> SPVAGQKYDYILVGGGTAACVLANRLSADGSKRVLVLEAGPDNTSRDVKIPAAITRLFRSPLDWNLFSELQEQLAERQIYMARGRLLGGSSATNATLYHRGAAGDYDAWGVEGWSSEDVLSWFVQAETNADFGPGAYHGSGGPMRVENPRYTNKQLHTAFFKAAEEVGLTPNSDFNDWSHDHAGYGTFQVMQDKGTRADMYRQYLKPVLGRRNLQVLTGAAVTKVNIDQAAGKAQALGVEFSTDGPTGERLSAELAPGGEVIMC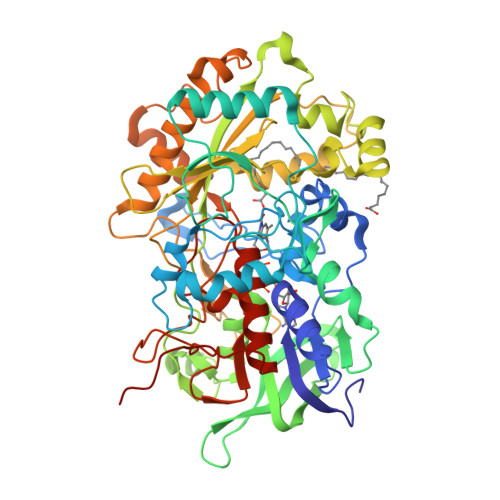AGAVHTPFLLKHSGVGPSAELKEFGIPVVSNLAGVGQNLQDQPACLTAAPVKEKYDGIAISDHIYNEKGQIRKRAIASYLLGGRGGLTSTGCDRGAFVRTAGQALPDLQVRFVPGMALDPDGVSTYVRFAKFQSQGLKWPSGITMQLIACRPQSTGSVGLKSADPFAPPKLSPGYLTDKDGADLATLRKGIHWARDVARSSALSEYLDGELFPGSGVVSDDQIDEYIRRSIHSSNAITGTCKMGNAGDSSSVVDNQLRVHGVEGLRVVDASVVPKIPGGQTGAPVVMIAERAAALLTGKATIGASAAAPATVAA GLCNAC(BETA1-4)-MURNAC(1,6-ANHYDRO)-L-ALA-GAMMA-D-GLU-MESO-A2PM-D-ALA | C37 H59 N7 O20 | 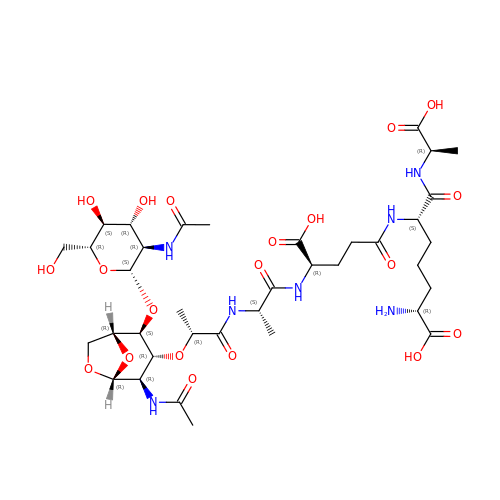UPFMKPIBAIPLHT-RSJSDIDPSA-N> MHHHHHHHHGGGGMHHPVAPVIDTVVNLAKRRGFVYPSGEIYGGTKSAWDYGPLGVELKENIKRQWWRSVVTGRDDVVGIDSSIILPREVWVASGHVDVFHDPLVESLITHKRYRADHLIEAYEAKHGHPPPNGLADIRDPETGEPGQWTQPREFNMMLKTYLGPIETEEGLHYLRPETAQGIFVNFANVVTTARKKPPFGIGQIGKSFRNEITPGNFIFRTREFEQMEMEFFVEPATAKEWHQYWIDNRLQWYIDLGIRRENLRLWEHPKDKLSHYSDRTVDIEYKFGFMGNPWGELEGVANRTDFDLSTHARHSGVDLSFYDQINDVRYTPYVIEPAAGLTRSFMAFLIDAYTEDEAPNTKGGMDKRTVLRLDPRLAPVKAAVLPLSRHADLSPKARDLGAELRKCWNIDFDDAGAIGRRYRRQDEVGTPFCVTVDFDSLQDNAVTVRERDAMTQDRVAMSSVADYLAVRLKGS

Glycyl tRNA synthetases (GlyRSs) are prospective drug targets for combating Mycobacterium tuberculosis (Mtb) and cancer in humans. Structures of all three forms – complete, or in some cases partial – have now been determined using X-ray diffraction or cryo-EM. Both Mycobacterial and human cells express the α2 subtype, and notably, the GlyRS gene in humans encodes one product that serves both the cytosol and mitochondria, which has obvious advantages for the design of selective inhibitors. Similar to the TtGlyRS, the two Mycobacterial GlyRS subunits adopt the canonical architecture consisting of an N-terminal catalytic domain and a C-terminal anticodon binding domain connected by a β-hairpin insertion. The catalytic core contains the class-II specific antiparallel β-sheet having the characteristic insertion domain after the first strand of the core β-sheet, and the anticodon recognition domain adopts the HGPT fold also found in HisRS, ProRS, and ThrRS.

In the present study, high-resolution crystal structures of MtbGlyRS and MtrGlyRS bound to glycyl-AMS were determined by X-ray diffraction to resolutions of 2.25 and 1.95 Å, respectively. To produce MtbGlyRS, the glyQS gene (with an N-terminal purification tag) was cloned into an M. smegmatis expression vector pDTCF and transformed into M. smegmatis, and expression of MtbGlyRS was induced by anhydrotetracycline. The present study describes the first crystal structures of bacterial class IIa GlyRSs bound to glycyl-AMS and magnesium, which closely recapitulate the binding site architecture of the glycyl-adenylate-bound TtGlyRS. The sulfamoyl group binds the guanidinium of Arg197 and ligates the divalent metal via its two oxygens; the nitrogen does not interact with the protein but instead forms a hydrogen bond with an active site water. In the glycyl group binding site, the carbonyl oxygen forms hydrogen bonds with both the Arg197 and Gln214 side chains. The amino group is held by the carboxylates of Glu216, Glu165, and Glu324. The configuration of the carboxylates, especially that of Glu324, together with the presence of the side chain of Ala326, impede the binding of pro S substituents, thus providing the molecular basis for the substrate specificity. In transitioning from the AMP to glycyl-AMS bound states, the largest conformational change involves closure of the lid motif, with displacements having magnitudes as great as 5.6 Å that accompany a twist in the central sheet. While the lid and glycyl-AMS lack close contacts, the hydroxyl group of Tyr264 is placed 3.6 Å from the electrophilic glycyl carbonyl carbon. In contrast to previously solved structures containing related ligands, the structures presented here also detail the magnesium coordination sphere.>MSQRITIDPVTRIQGHLRIDCEIENGVVSKAWASGTMWRGMEEIVKNRDPRDAWMIVQRICGVCTTTHALSSVRAAESALNIDVPVNAQYIRNIILAAHTTHDHIVHFYQLSALDWVDITSALQADPTKASEMLKGVSTWHLNSPEEFTKVQNKIKDLVASGQLGIFANGYWGHPAMKLPPEVNLIAVAHYLQALECQRDANRVVALLGGKTPHIQNLAVGGVANPINLDGLGVLNLERLMYIKSFIDKLSDFVEQVYKVDTAVIAAFYPEWLTRGKGAVNYLSVPEFPTDSKNGSFLFPGGYIENADLSSYRPITSHSDEYLIKGIQESAKHSWYKDEAPQAPWEGTTIPAYDGWSDDGKYSWVKSPTFYGKTVEVGPLANMLVKLAAGRESTQNKLNEIVAIYQKLTGNTLEVAQLHSTLGRIIGRTVHCCELQDILQNQYSALITNIGKGDHTTFVKPNIPATGEFKGVGFLEAPRGMLSHWMVIKDGIISNYQAVVPSTWNSGPRNFNDDVGPYEQSLVGTPVADPNKPLEVVRTIHSFDPCMACAVHVVDADGNEVVSVKVL[2x];>EMAESVTNPQRPPVIWIGAQECTGCTESLLRATHPTVENLVLETISLEYHEVLSAAFGHQVEENKHNALEKYKGQYVLVVDGSIPLKDNGIYCMVAGEPIVDHIRKAAEGAAAIIAIGSCSAWGGVAAAGVNPTGAVSLQEVLPGKTVINIPGCPPNPHNFLATVAHIITYGKPPKLDDKNRPTFAYGRLIHEHCERRPHFDAGRFAKEFGDEGHREGWCLYHLGCK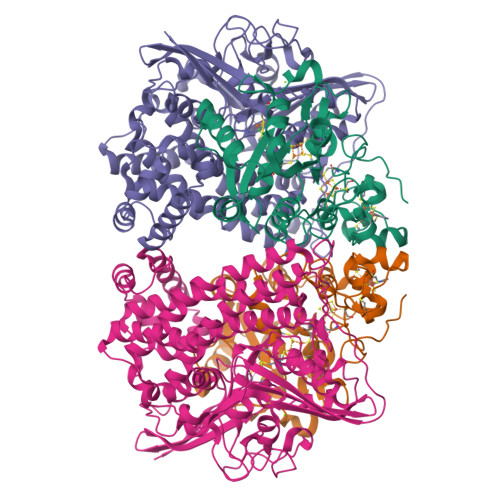GPETYGNCSTLQFCDVGGVWPVAIGHPCYGCNEEGIGFHKGIHQLANVENQTPRSQKPDVNAKEGGRSHHHHHH[2x]Glucuronoyl esterases (GEs) from carbohydrate esterase family 15 (CE15) have been suggested to play key roles in reducing lignocellulose recalcitrance by cleaving covalent ester bonds found between lignin and glucuronoxylan. The enzymes are α/β-hydrolases with a catalytic triad typical of esterases. The targets, exhibiting sequence identities as low as 25%, were biochemically characterized using a range of model substrates, and the three-dimensional structures were solved for two of the enzymes. The structural determinations of OtCE15A and SuCE15C reveal similar overall folds to previously determined CE15 structures, with closest structural similarity to the recently released bacterial structure of MZ0003.

Like MZ0003, Reg2 in OtCE15A and SuCE15C comprises 40–45 residues originating from β4 and contains a few short helical segments and, in the case of SuCE15C, two β strands which form a slightly misaligned antiparallel sheet. The tryptophan residue in StGE2 (Trp310) found hydrogen bonding to the 2-OH of the ligand is conserved in the bacterial structures (Trp358 in OtCE15A, Trp348 in SuCE15C, and Trp334 in MZ003), whereas Glu267 in StGE2 which hydrogen bonds with both 2-OH and the anomeric hydroxyl group (in β configuration) is not conserved (Arg303 in SuCE15C, Val313 in OtCE15A, and Ser289 in MZ0003). Gln259 of StGE2 is observed hydrogen bonding with both the 2-OH and 3-OH moieties of the sugar ring, and the equivalently positioned residues (with respect to main chain) in OtCE15A, SuCE15C, and MZ0003 are Glu305, Glu295, and Glu281, respectively. However, in SuCE15C, the loop containing Glu295 is modeled with the acidic side chain rotated away from the active site, and instead Arg296 occupies the equivalent space. In the bacterial structures, small residues are found in the equivalent leucine position (Ala359 in OtCE15A, Ser349 in SuCE15C, and Ala335 in MZ0003) while an aspartate residue is found in the same position as the isoleucine (Asp356 in OtCE15A, Asp346 in SuCE15C, and Asp332 in MZ0003). A small cleft within the pocket formed by Reg2 contains a conserved phenylalanine residue (Phe141 in OtCE15A, Phe135 in SuCE15C, and Phe117 in MZ0003) and a basic residue (Lys183 in OtCE15A, Arg173 in SuCE15C, and Arg160 in MZ0003). Three of the enzymes, OtCE15D, SuCE15A & C, exhibited exceptionally high catalytic efficiencies (in the 104 s−1 M−1 range) on BnzGlcA, which is 10 to 100-fold higher than reported for fungal GEs. SuCE15C was consistently the most efficient boosting enzyme, followed by SuCE15A and SlCE15A, somewhat reflecting their activity levels on BnzGlcA. To investigate putative lignin- and xylan-binding sites in our solved structures, docking simulations of OtCE15A and SuCE15C with a benzyl ester of 4-O-methyl-glucuronoxylotriose (glucuronoate α-1,2 linked to the middle xylose residue) were performed.

> GHITDEAKVPAYTLPAVLALKSGQPVTDAKSWTTKRRPEILAIYEAEVYGKSPARPPKLNYEVKSVEKQALGGKATRKIVTIFFSDKPDAPKMDLLLYLPAAAAKPAPVILGLSFGGIHTVANDPGVPLAEQWTRDNRKQPSAEKSRGGEASRWQVEKILAAGYGLATVYYEQIEPDFAGGMKYGIRPLFFKPGQTEPEPGDWGAVAAWAWGASRAMDYLEKDKDVDARRVGLIGHSRLGKAAIWAGAQDARFTFIISNESGEGGAAISRRDYGERTTALNTRFPHWFDGNYKKYNDRENEMPFDSHMALALMAPRGLYVASAEGDQWSDPKGEFLGAANASPVWELFGKKGIGTMTMPDLHEPVGDSVRYHIRAGKHDVTEYDWEQYLKFAKAQWG>SNAMNIKTVEDLFIHLLSDTYSAE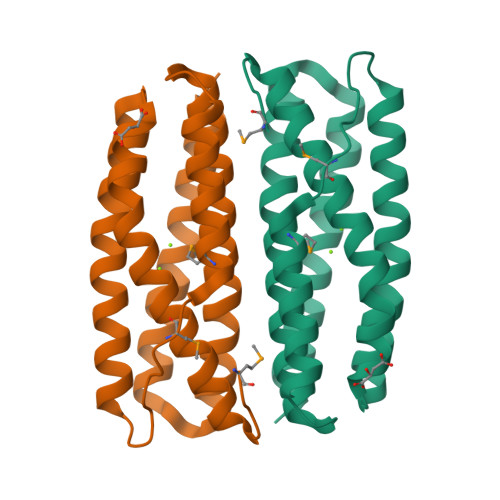KQLTKALPKLARATSNEKLSQAFQSHLEETQGQIERIDQIVESESGIKLKRMKCVAMEGLIEEANEVIESTEKNEVRDAALIAAAQKVEHYEIASYGTLATLAEQLGYSKALKLLKETLDEEKQTDLKLTDLAVSNVNKSAERKSK[2x]> MAAHHRQNTAGRRKVQVSYVIRDEVEKYNRNGVNALQLDPALNRLFTAGRDSIIRIWSVNQHKQDPYIASMEHHTDWVNDIVLCCNGKTLISASSDTTVKVWNAHKGFCMSTLRTHKDYVKALAYAKDKELVASAGLDRQIFLWDVNTLTALTASNNTVTTSSLSGNKDSIYSLAMNQLGTIIVSGSTEKVLRVWDPRTCAKLMKLKGHTDNVKALLLNRDGTQCLSGSSDGTIRLWSLGQQRCIATYRVHDEGVWALQVNDAFTHVYSGGRDRKIYCTDLRNPDIRVLICEEKAPVLKMELDRSADPPPAIWVATTKSTVNKWTLKGIHNFRASGDYDNDCTNPITPLCTQPDQVIKGGASIIQCHILNDKRHILTKDTNNNVAYWDVLKACKVEDLGKVDFEDEIKKRFKMV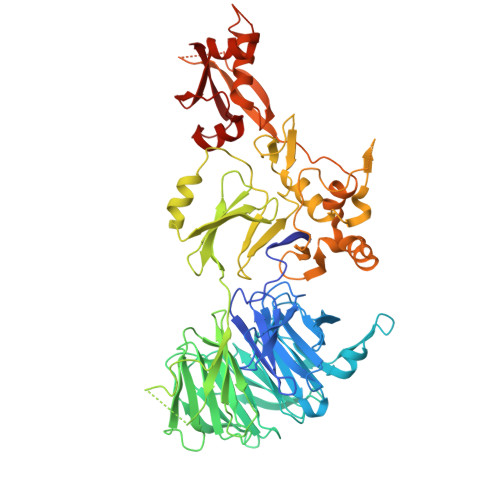YVPNWFSVDLKTGMLTITLDESDCFAAWVSAKDAGFSSPDGSDPKLNLGGLLLQALLEYWPRTHVNPMDEEENEVNHVNGEQENRVQKGNGYFQVPPHTPVIFGEAGGRTLFRLLCRDSGGETESMLLNETVPQWVIDITVDKNMPKFNKIPFYLQPHASSGAKTLKKDRLSASDMLQVRKVMEHVYEKIINLDNESQTTSSSNNEKPGEQEKEEDIAVLAEEKIELLCQDQVLDPNMDLRTVKHFIWKSGGDLTLHYRQKST>MLTVDLSGKKALVMGVTNQRSLGFAIAAKLKEAGAEVALSYQAERLRPEAEKLAEALGGALLFRADVTQDEELDALFAGVKEAFGGLDYLVHAIAFAPREAMEGRYIDTRRQDWLLALEVSAYSLVAVARRAEPLLREGGGIVTLTYYASEKVVPKYNVMA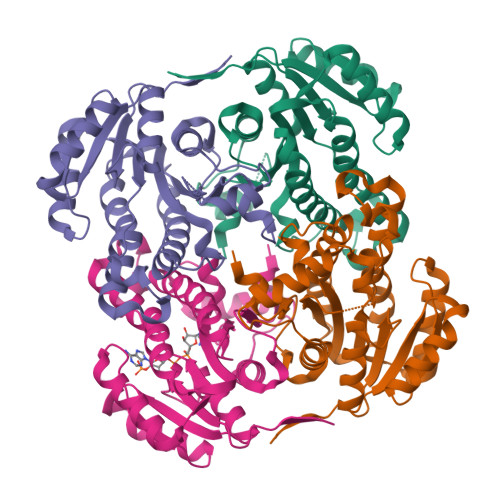IAKAALEASVRYLAYELGPKGVRVNAISAGPVRTVAARSIPGFTKMYDRVAQTAPLRRNITQEEVGNLGLFLLSPLASGITGEVVYVDAGYHIMGMELEG[8x]> MSIDLKKRKVEEDVRSRGKNSKIFSPFRIIGN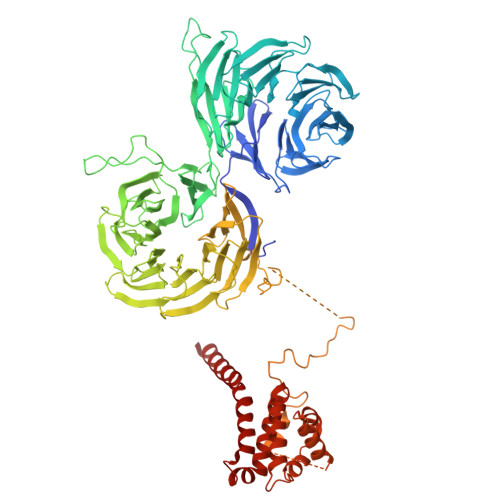VSNGVPFATGTLGSTFYIVTCVGKTFQIYDANTLHLLFVSEKETPSSIVALSAHFHYVYAAYENKVGIYKRGIEEHLLELETDANVEHLCIFGDYLCASTDDNSIFIYKKSDPQDKYPSEFYTKLTVTEIQGGEIVSLQHLATYLNKLTVVTKSNVLLFNVRTGKLVFTSNEFPDQITTAEPAPVLDIIALGTVTGEVIMFNMRKGKRIRTIKIPQSRISSLSFRTDGSSHLSVGTSSGDLIFYDLDRRSRIHVLKNIHRESYGGVTQATFLNGQPIIVTSGGDNSLKEYVFDPSLSQGSGDVVVQPPRYLRSRGGHSQPPSYIAFADSQSHFMLSASKDRSLWSFSLRKDAQSQEMSQRLHKKQDGGRVGGSTIKSKFPEIVALAIENARIGEWENIITAHKDEKFARTWDMRNKRVGRWTFDTTDDGFVKSVAMSQCGNFGFIGSSNGSITIYNMQSGILRKKYKLHKRAVTGISLDGMNRKMVSCGLDGIVGFYDFNKSTLLGKLKLDAPITAMVYHRSSDLFALALDDLSIVVIDAVTQRVVRQLWGHSNRITAFDFSPEGRWIVSASLDSTIRTWDLPTGGCIDGIIVDNVATNVKFSPNGDLLATTHVTGNGICIWTNRAQFKTVSTRTIDESEFARMALPSTSVRGNDSMLSGALESNGGEDLNDIDFNTYTSLEQIDKELLTLSIGPRSKMNTLLHLDVIRKRSKPKEAPKKSEKLPFFLQLSGEKVGDEASVREGIAHETPEEIHRRDQEAQKKLDAEEQMNKFKVTGRLGFESHFTKQLREGSQSKDYSSLLATLINFSPAAVDLEIRSLNSFEPFDEIVWFIDALTQGLKSNKNFELYETFMSLLFKAHGDVIHANNKNQDIASALQNWEDVHKKEDRLDDLVKFCMGVAAFVTTA> GPLGSVRDEIRSMVSDSVDEIVDGVSKTTAEVINGRKSIAQYATSLIESNPEPDNVRTIISQPLIKNTFLLVGFGLEKDGSNINNDPSWNPGPTWDPRVRPWYKDAKNAGKLVITAPYADSASGEILVSVATPVKDSATGQFLGSIFYDVSLAELAELVNEVKLFDAGYVFIVSEDGTTIAHPKKEFNGKPMSEFLGESKINVDTHQVIINGKPYAVSFSDVEGEDWYVGVVIDEEIAYAALDELRRSTLIHHHHHH

Extracellular signals are sensed by methyl-accepting chemotaxis proteins (MCPs), also known as chemoreceptors. Indeed, we found that Mlp37, the closest homolog of Mlp24, serves as a chemoreceptor for taurine as well as serine, arginine and other amino acids. We determined the crystal structures of the ligand-binding domain of Mlp37 in complex with l-serine and taurine to reveal the molecular mechanism enabling Mlp37 to accommodate these structurally distinct ligands, l-serine and taurine. The ligand complex structures and the mutational analyses demonstrate that only one of the two potential ligand-binding pockets (the membrane-distal pocket I) is involved in ligand binding by Mlp37.

In contrast, the l-serine complex forms a dimer with a molecule related by crystallographic two-fold symmetry. Taurine and l-serine are bound only in pocket I in the crystal structures. The amino group of l-serine is in contact with Tyr-170, Asp-201 and Asp-172, which are triangularly arranged around it. The carboxyl group of l-serine interacts mainly with the guanidino group of Arg-152. The indole NH of Trp-154 and the main-chain amino group of Ser-173 also contribute to the binding of the carboxyl group of the l-serine ligand. The side-chain hydroxyl group of l-serine is recognised by Asp-172 and the indole NH of Trp-141. As a result, the entrances to pocket I in the l-serine and taurine complexes are slightly open. Such an opening would allow larger amino acid R groups of other amino acids to stick out from the pocket without significantly affecting interactions with the amino acid backbone atoms, a situation that could explain the ability of Mlp37 to sense a diversity of amino acids. The l-serine complex, in which the hydroxyl group of the ligand points toward the small opening of pocket I, reveals the molecular basis for the diversity of amino acids that can be sensed by Mlp37. The slightly open conformation of pocket I in the serine complex enabled us to visualise ligand binding in vivo with a fluorescently labelled amino acid.>CKFKFQF[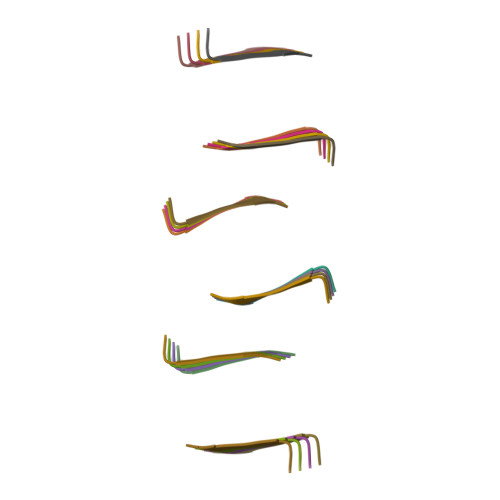24x]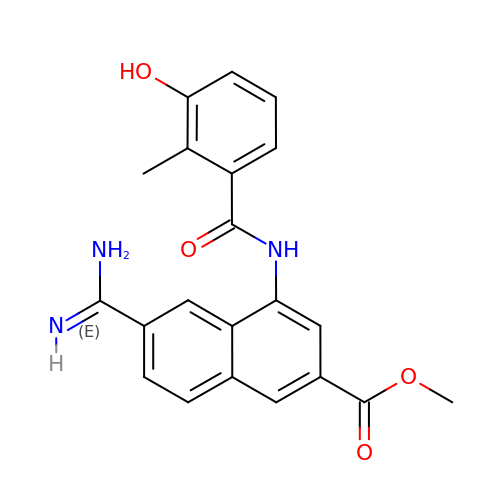6-CARBAMIMIDOYL-4-(3-HYDROXY-2-METHYL-BENZOYLAMINO)-NAPHTHALENE-2-CARBOXYLIC ACID METHYL ESTER | C21 H19 N3 O4 | OUBRALHIKGRAMA-UHFFFAOYSA-N3-[[(METHYLAMINO)SULFONYL]AMINO]-2-OXO-6-PHENYL-N-[3,3,3-TRIFLUORO-1-(1-METHYLETHYL)-2-OXOPHENYL]-1(2H)-PYRIDINE ACETAMIDE | C20 H23 F3 N4 O5 S | 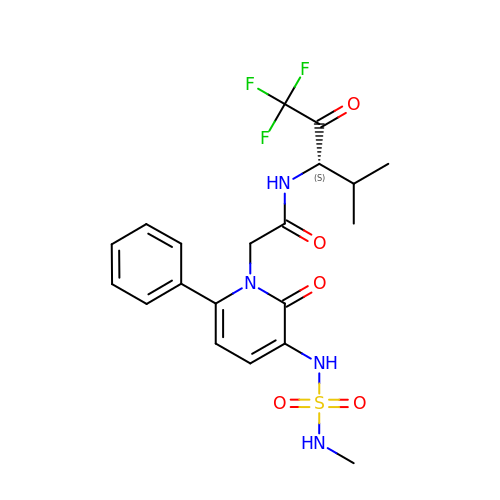MYFMPKCOIMRDDD-KRWDZBQOSA-N>AAGRRGSFVEMVDNLRGKSGQGYYVEMTVGSPPQTLNILVDTGSSNFAVGAAPHPFLHRYYQRQLSSTYRDLRKGVYVPYTQGKWEGELGTDLVSIPHGPNVTVRANIAAITESDKFFINGSNWEGILGLAYAEIARPDDSLEPFFDSLVKQTHVPNLFSLQLCGAGFPLNQSEVLASVGGSMIIGGIDHSLYTGSLWYTPIRREWYYEVIIVRVEINGQDLKMDCKEYNYDKSIVDSGTTNLRLPKKVFEAAVKSIKAASSTEKFPDGFWLGEQLVCWQAGTTPWNIFPVISLYLMGEVTNQSFRITILPQQY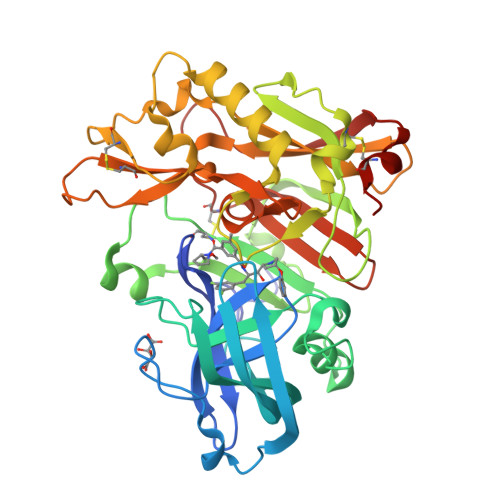LRPVEDVATSQDDCYKFAISQSSTGTVMGAVIMEGFYVVFDRARKRIGFAVSACHVHDEFRTAAVEGPFVTLDMEDCGYNI[2x]3,4-dihydroquinazolin-4-ol | C8 H8 N2 O | 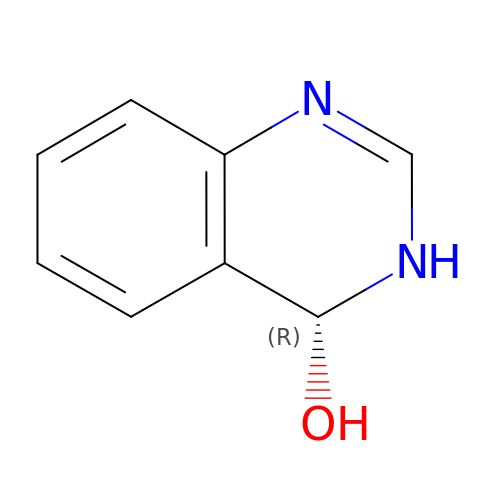RFXUVQZRJWPTLS-MRVPVSSYSA-N> MTLNRKCVVIHNGSHRTVAGFSNVELPQCIIPSSYIKRTDEGGEAEFIFGTYNMIDAAAEKRNGDEVYTLVDSQGLPYNWDALEMQWRYLYDTQLKVSPEELPLVITMPATNGKPDMAILERYYELAFDKLNVPVFQIVIEPLAIALSMGKSSAFVIDIGASGCNVTPIIDGIVVKNAVVRSKFGGDFLDFQVHERLAPLIKEENDMENMADEQKRSTDVWYEASTWIQQFKSTMLQVSEKDLFELERYYKEQADIYAKQQEQLKQMDQQLQYTALTGSPNNPLVQKKNFLFKPLNKTLTLDLKECYQFAEYLFKPQLISDKFSPEDGLGPLMAKSVKKAGASINSMKANTSTNPNGLGTSHINTNVGDNNSTASSSNISPEQVYSLLLTNVIITGSTSLIEGMEQRIIKELSIRFPQYKLTTFANQVMMDRKIQGWLGALTMANLPSWSLGKWYSKEDYETLKRDRKQSQATNATN;> MAPFRQDSILIIYPRSQTTLVQFGLNEETFTVPELEIPTQIYRTTRQDGSYTYHSTNKDNKAELIKPIQNGEIIDISAFTQFLRLIFVSILSDRANKNQDAFEAELSNIPLLLITHHSWSQSDLEIITQYVFESLEINNLIQLPASLAATYSMISLQNCCIIDVGTHHTDIIPIVDYAQLDHLVSSIPMGGQSINDSLKKLLPQWDDDQIESLKKSPIFEVLSDDAKKLSSFDFGNENEDEDEGTLKNSDLEFNTFWDEKGNEIKVGKQRFQGCNNLIKNISNRVGLTLDNIDDINKAKAVWENIIIVGGTTSISGFKEALLGQLLKDHLIIEPEEEKSKREEEAKSVLPAATKKKSKFMTNSTAFVPTIEYVQCPTVIKLAKYPDYFPEWKKSGYSEIIFLGAQIVSKQIFTHPKDTF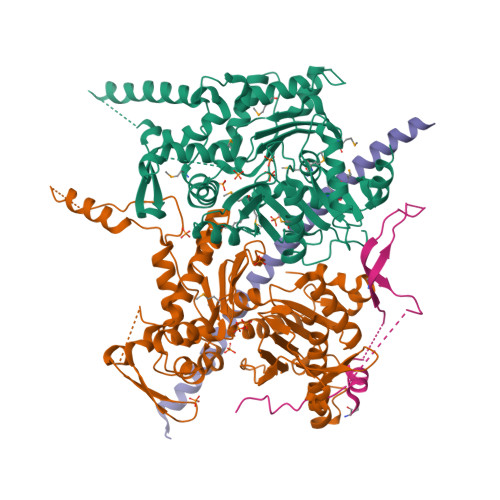YITREKYNMKGPAALWDVQF;> MGHHHHHHHHHHGNVQDALLTNQLYKNHELLKLERKKTEAVARLKSMNKSAINQYNRRQDKKNKRLKFGHRLIATHTNLERDEQKRAEKKAKERLQALKANDEEAY;> MDPQTLITKANKVSYYGNPTSKESWRYDWYQPSKVSSNVQQPQQQLGDMENNLEKYPFRYKTWLRNQEDEKNLQRESCEDILDLKEFDRRILKKSLMTSHTKGDTSKATGAPSANQGDEALSVDDIRGAVGNSEAIPGLSAGVNNDNTKESKDVKMN> ADTRIGVTIYKYDDNFMSVVRKAIEQDAKAAPDVQLLMNDSQNDQSKQNDQIDVLLAKGVKALAINLVDPAAAGTVIEKARGQNVPVVFFNKEPSRKALDSYDKAYYVGTDSKESGIIQGDLIAKHWAANQGWDLNKDGQIQFVLLKGEPGHPDAEARTTY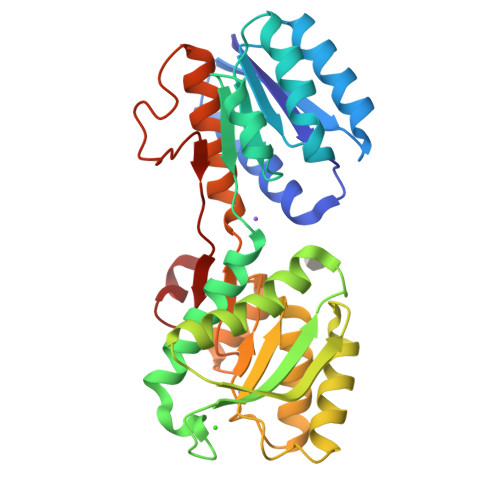VIKELNDKGIKTEQLQLDTAMWDTAQAKDKMDAWLSGPNANKIEVVIANNDAMAMGAVEALKAHNKSSIPVFGVDALPEALALVKSGALAGTVLNDANNQAKATFDLAKNLADGKGAADGTNWKIDNKVVRVPYVGVDKDNLAEFSKK Here, we report on the structural determination of PorX, a noncanonical RR that comprises a classic REC domain and an additional enzymatic effector domain that exhibits phosphodiesterase activity. Our crystal structures reveal that the PorXFJ adopts a two-domain dimeric fold with a classical RR receiver domain's fold and a unique alkaline phosphatase superfamily (APS) domain connected by a helical linker region. Each PorXFJ monomer adopts a two-lobed fold containing an N-terminal receiver (REC) domain (residues 1–120), followed by a three-helix bundle (THB) domain (residues 121–209) and a C-terminal APS domain (residues 210–517). All PorXFJ dimers adopt an intertwined assembly, where each monomer is symmetrically wrapped around the other monomer, forming an overall “X”-like shape.

Among the different orthologues screened, we identified two distinctive conditions promoting the crystallization of the full-length PorX from F. johnsoniae (PorXFJ) in its nonphosphorylated apo-form. Heavy-atom derivative (bromide) soaking, followed by a multiwavelength anomalous diffraction data collection, were used to retrieve the missing phase information and solve the high-resolution structure of PorXFJ. Although the purified nonphosphorylated PorXFJ was found to be monomeric in solution by size exclusion chromatography, both crystal forms presented an identical dimeric assembly within their asymmetric units. The primitive orthorhombic crystal form gave rise to a single dimeric assembly (two monomers in the asymmetric unit), while the primitive monoclinic crystal form gave rise to two identical dimeric assemblies (four monomers in the asymmetric unit). In the primitive orthorhombic crystal form, residues 358–369 adopt a helical conformation in one monomer while presenting an extended coil conformation and an additional helical turn at the N terminal of helix α16 in the second monomer. Global comparison of the APS dimerization interface demonstrates that the 358–369 helical-extended coil conformation dyad gives rise to a total of 1,080 Å2 surface area, while the helical–helical conformations dyad interface is only 993 Å2, suggesting the helical-extended loop conformation to be more stable. In particular, only the helical conformation of residues 358–369 can support the proper coordination of the Zn1 by the conserved Asp360 and His364 residues, whereas in the extended coil conformation, these residues are facing away from the APS catalytic site.

>[2x]GSHMDKIRILWVDDEIDLLKPHILFLEKKNYEVTTSNNGLDAIALFEEENFDIVFLDENMPGMSGLETLSEMKEKKSAIPMIMITKSEEEYIMEEAIGSKIADYLIKPVNPNQILLSLKKNLDDSRLITEKTTLDYQKEFRKISMELAMVNSYEDWVELYKKLLFWELKLEDINDQAMIEILESQKVEANSQFGKYIERNYEDWFAPKADKPIQSHNLFKELVVPEIKKKDKPILFVVIDNLRYDQWKSFETVISNYYKLEKEVPYFSILPTATQYARNAIFSGLMPLDMEKQFPQYWKNDVEDGGKNLYEAEFLSAQIKRLGLNIKEDYFKITNYAGGKKLAENFKALKGNDLVTVVYNFVDMLSHAKTEMEVVKELASDDKAYRSLTLSWFKNSPLLEIIQQAQLLGFKLILTTDHGTINVKNPSKVVGDKNTSLNLRYKTGRSLTYEQKDVYVVKEPKTIGLPAINMSSSFIFAKNDFFLAYVNNYNHYVSYYKNTYQHGGISLEEMIIPFLVFNPK>GPGSMNGISVEHDGAVLRIRLDRPEKLNAVDTPMLEELSVHIRDAEADESVRAVLLTGAGRAFCSGGDLTGGDTAGAADAANRVVRAITSLPKPVIAGVHGAAVGFGCSLALACDLVVAAPASYFQLAFTRVGLMPDGGASALLPLLIGRARTSRMAMTAE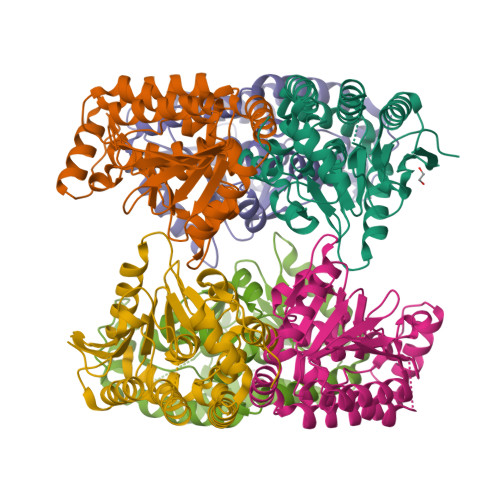KISAATAFEWGMISHITSADEYESVLTDVLRSVSGGPTLAFGWTKRALAAATLAELEPVQAIEAEGQLALVETADFREGARAFRERRTPNFRGH[6x]> SMNPPAGPVRAIAEYERSAAVLVRYPFGIPMELIKELAKNDKVITIVASESQKNTVITQYTQSGVNLSNCDFIIAKTDSYWTRDYTGWFAMYDTNKVGLVDFIYNRPRPNDDEFPKYEAQYLGIEMFGMKLKQTGGNYMTDGYGSAVQSHIAYTENSSLSQAQVNQKMKDYLGITHHDVVQDPNGEYINHVDCWGKYLAPNKILIRKVPDNHPQHQALEDMAAYFAAQTCAWGTKYEVYRALATNEQPYTNSLILNNRVFVPVNGPASVDNDALNVYKTAMPGYEIIGVKGASGTPWLGTDALHARTHEVADKGYLYIKHYPILGEQAGPDYKIEADVVSCANATISPVQCYYRINGSGSFKAADMTMESTGHYTYSFTGLNKNDKVEYYISAADNSGRKETYPFIGEPDPFKFTCMNETNTCTVTGAAKALRAWFNA

To this end, citrullination by the only known prokaryotic PAD expressed by keystone periodontal pathogen Porphyromonas gingivalis (PPAD) has been implicated in the aetiology of RA. PPAD is organised into four domains: the N-terminal signal peptide (NtSP, aa 1-48), catalytic/deiminase domain (CD, aa 49-360), Ig-like fold (IgLF, aa 361-463) and C-terminal domain (CTD, aa 464-556). The CD adopts the canonical fold of ββαβ motifs conserved among GME structures (RMSD 2.0–2.4 Å). The PPAD active site is an elongated cavity with its entrance exposed to the surface exterior.

An equivalent mutant construct (tPPADC351A) with the essential catalytic nucleophile among GMEs Cys35126 substituted to Ala, is catalytically inactive. We have determined the 1.46 Å and 1.48 Å structures of tPPADWT and tPPADC351A by molecular replacement, which reveal identical and superimposable conformations (root mean square deviation (RMSD)∼0.09 Å), suggesting that the Cys351Ala substitution did not perturb protein integrity. Difference Fourier electron density maps clearly reveal an active site-bound ligand, modelled in the tPPADC351A structure as an arginine-containing dipeptide, and in the tPPADWT structure as an amidino adduct where its Cζ atom is covalently linked to the Cys351 S atom. The tPPADC351A structure captures an intact arginine side chain without enzymatic turnover, mimicking the enzyme-substrate Michaelis complex prior to catalysis. At the end of the cavity, the site of the PPAD citrullination reaction, both ligands are coordinated by five polar residues strictly conserved among GMEs, namely Asp130, His236, Asp238, Asn297 and Cys351/Ala351. Located away from the site of nucleophilic attack, Arg152 and Arg154 form ionic bonds with the free carboxyl group of a C-terminal arginine, stabilising the substrate for enzymatic turnover. Citrullination activity of tPPADWT on FibA-R was significantly higher than FibA-R-XX (p=0.003), the latter equivalent to the baseline measurement level for inactive tPPADC351A. The crystallised tPPADWT and tPPADC351A constructs include residues aa464–484, with no visible electron density. This region represents a flexible linker connecting the IgLF and CTD in the full-length polypeptide, and its flexibility likely caused disorder in the crystal.>[2x]GPGIPPKIEALPSDISIDEGKVLTVACAFTGEPTPEVTWS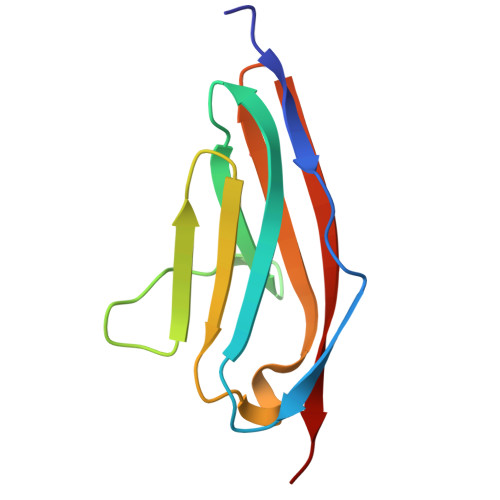CGGRKIHSQEQGRFHIENTDDLTTLIIMDVQKQDGGLYTLSLGNEFGSDSATVNIHIRSI4-methyl-3-[(1-methyl-6-pyrazin-2-yl-pyrazolo[3,4-d]pyrimidin-4-yl)amino]-~{N}-[3-(trifluoromethyl)phenyl]benzamide 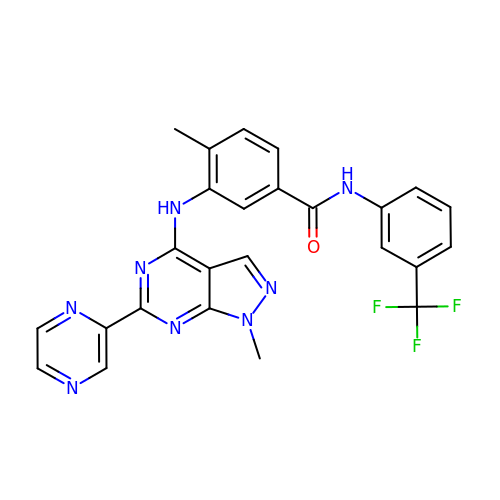| C25 H19 F3 N8 O | NPNYLZWEJSSGBG-UHFFFAOYSA-N>MLEQMISSSKVGVKINEWYKYIRLFSVPDSEILKAEVEEEIRHMKEDHDLLLYYSLMCFRHQLMLDYLEPKTLNEERPKISDLLEKIESSQTDLKGILEYYFNFFRGMYEFEQYEYLNAISFYKQAERKLSLVADEIERAEFHYKVAEIYYHMKQTHMSMHHIVQAIDSYKAHENYTVRVIQCSFVIGLNYLDMDYPEKAIPHFKNALDKAREIDMSRLIGSSLYNLGLCSFAEEAYEKASEYFKEGIRVYQDNGYEHSNRILDILLMLTKTTFKMRNHSEGISWCAHGLSLSKNLNDEIMAKMFEFIHALYVDNDNEKLNSILN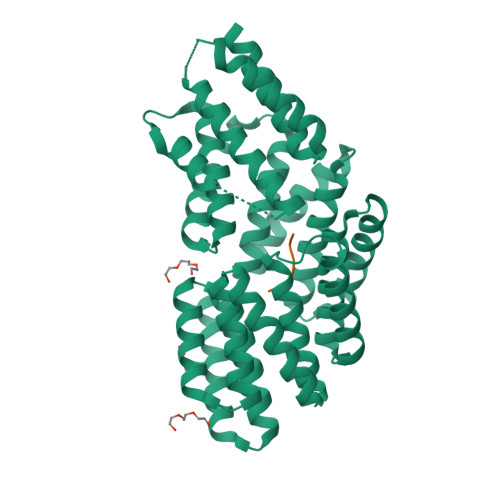YLELKSMLSDVEDLASDAAKYYNEKEDHKVAVAYYEKVLYARKQIQRGDCLYET[2x];>[2x]RGHTS> MIYTTDKEFKKNLENALAHVYSTQIENSAPDQVEFRKVAWLRLKDMLYNQLLDKNLPAKINGYDPGLMETISPTQPQHIIPHLVKMNKIDQLIWKKITGKTEGVTKYEQFQYLLSSYYDCILNQEIIPSMLNTGTDDSVHSVDFSNPAEWFPEARKIRRHIIMHVGPTNSGKTFRSLQKLKAADRGYYAGPLRLLAREVYEKFKHENVRCNLLTGEEVIKDLDEM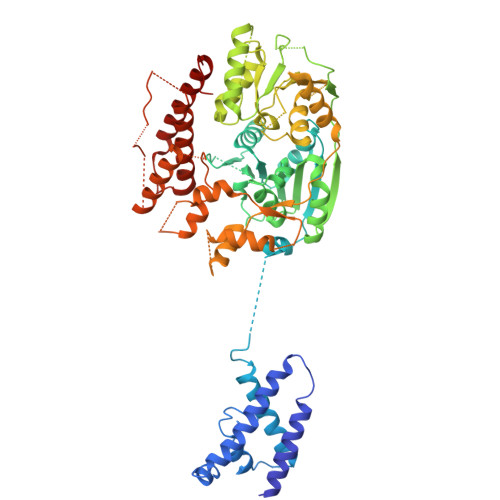GNEANLTSGTIEMIPLNQNFDVVVLDEIQMMADLDRGWAWTNALLGAKAKEVHCCGEASTIPLIKKIVEMTGDKLTINEYERMGKLVVEEEALTKGYHSLKKGDCVVAFSKKAILDLKLEIEKKTELKAAVIYGSLPPETRVKQANLFNSGEFDILIASDAIGMGLNLSIDRVVFTTSKKFDGRDMVDMTSSAIKQIGGRAGRFKQNIHDNGELPVGYITAVKPNVLKAVREAINAPIEYLTSATTWPTDEICTHVMTRFMPGTTCKTLLETIAADIEQSSNKLFQICDLKARMSAIEIIDSMEDITFSDKLRLSNAPLKDFPLVKAAFKKFCDTIARGHTRGLLSYRFPFDILNLKYIYTEKHGLEEYEALYNIIMLFFWLSNRYPNYFIDQESASELKNFCEMIIFEKIDHLKRNPY HIV-1 Nef is an important accessory protein that is attributed with multiple distinct functions such as immune evasion, virion infectivity and support for viral replication and survival. Each Nef chain folds into two domains. The C-terminal core-domain functions as the oligomerization and protein interaction domain. It contains the PXXP motif (Residues 72–78) that recognizes SH3 domains of partner proteins and other interaction motifs at a 30-residue loop (Residues 149–178) distal to the PXXP motif.

We report the crystallization of the full-length HIV-1 Nef after experimentation with naturally occurring Nef variants from patient samples and were successful with one such sample. The protein adopts the elusive closed tetrameric association in the structure. The asymmetric unit contains two protein chains that associate through symmetry to form a tetramer. Surprisingly, the tetramer exhibits 4-fold symmetry as opposed to a normally expected 222 symmetry when two dimers associate together. On the other hand, the N-terminal anchor domain is disordered in the full-length structure. Compared to the dimeric association of the earlier ‘open’ form, one subunit of the core-domain swings out with a relative rotation of about 174° and translation by ∼22 Å with respect to the respective center of masses. Further association with another symmetric pair leads to the formation of the tetramer. This leads to the steric shielding of the PXXP motif in the tetramer. The Arg105 of the earlier Nefcore structure is the first residue of the conserved XR motif, where X is either R or K. In the tetrameric association the Asp125 (Asp123 of Nefcore structure) now interacts with the second R residue of the XR motif. Thus the Nef tetramer can selectively abrogate the recognition of SH3 domains while allowing for interactions with other subsets of its repertoire of protein partners.

> MGGKWSKSSIVGWPAIRERLRRAQPAAERRRAQPAAEGVGAASQDLGRHGALTSSNTDTTNADEEEEVGFPVRPQVPLRPMTYKGAVDLSFFLKEKGGLEGLVYSQREKEILDLWVYHTQGYFPDWQCYTPGPGVRYPLTFGWCFKLVPVDPGEVEEATEGENNCLLHPICQHGMDDDHREVLKWKFDSHLAHTHMARELHPEYFKNC;> MGGKWSKSSIVGWPAIRERLRRAQPAAERRRAQPAAEGVGAASQDLGRHGALTSSNTDTTNADEEEEVGFPVRPQVPLRPMTYKGAVDLSFFLKEKGGLEGLVYSQKRKEILDLWVYHTQGYFPDWQCYTPGPGVRYPLTFGWCFKLVPVDPGEVEEATEGENNCLLHPICQHGMDDDHREVLKWKFDSHLAHTHMARELHPEFYKNC> IPITVDFSGGLEMLFDNQRRHSISLPAKDTEGKPVTIAFLIDYICKKL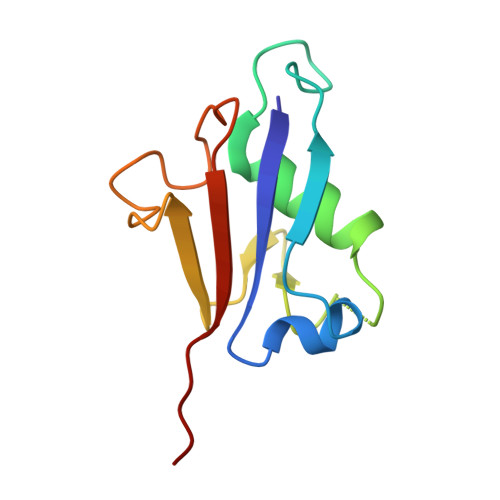MKDPRTDLFVLDNHIRPGILVLINDADWELEGEEAYEIQPNDNILFVSTLHGG> SPDTSVDNKVNFSTDVIYQIVTDRFADGDRTNNPAGDAFSGDRSNLKLYFGGDWQGIIDKINDGYLTGMGVTALWISQPVENITSVIKYSGVNNTSYHGYWARDFKQTNDAFGDFADFQNLIDTAHAHNIKVVIDFAPNHTSPADRDNPGFAENGALYDNGSLLGAHSNDTAGLFHHNGGTDFSTIEDGIYKNLYDLADINHNNNAMDAYFKSAIDLWLGMGVDGIRFDAVKHMPFGWQKSFVSSIYGGDHPVFTFGEWYLGADQTDGDNIKFANESGMNLLDFEYAQEVREVFRDKTETMKDLYEVLASTESQYDYINNMVTFIDNHDMDRFQVAGSGTRATEQALALTLTSRGVPAIYYGTEQYMTGDGDPNNRAMMTSFNTGT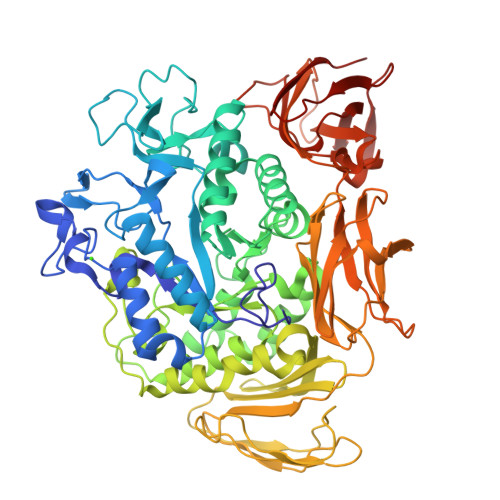TAYKVIQALAPLRKSNPAIAYGTTTERWVNNDVLIIERKFGSSAALVAINRNSSAAYPISGLLSSLPAGTYSDVLNGLLNGNSITVGSGGATTNFTLAAGGTAVWQYTAPETSPAIGNVGPTMGQPGNIVTIDGRGFGGTAGTVYFGTTVVTGSGIVSWEDTQIKAVIPKVAAGKTGVSVKTSSGTASNTFKSFNVLTGDQVTMRFLVNQANTNYGTNVYLVGNAAELGSWDPNKAIGPMYNQVIAKYPSWYYDVSVPAGTKLDFKFIKKGGGTVTWEGGGNHTYTTPASSVGTVTVDWQN>MGSHHHHHHSAALEVLFQGPGGNGKLRQWLIDQIDSGKYPGLVWENEEKSIFRIPWKHAGKQDYNREE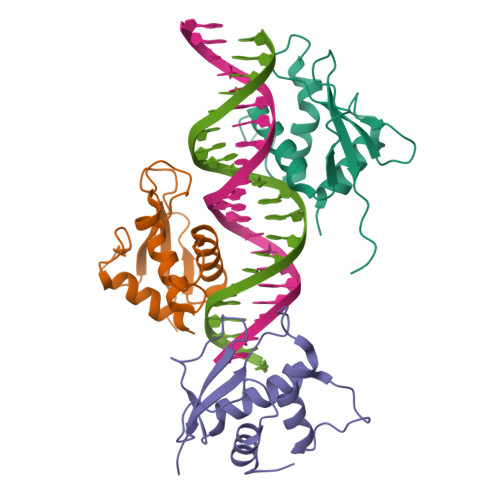DAALFKAWALFKGKFREGIDKPDPPTWKTRLRCALNKSNDFEELVERSQLDISDPYKVYRIVPEGAKKGAKQL[3x]>[3x]MHKSAFQALQGDIPTYEVNSSDEQDSDQDEEDVEQPSEPMHRLVSAPAASIHIEESKYISSNFSFDDD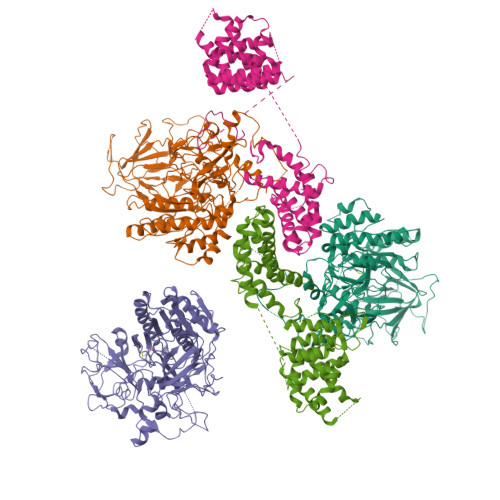NTIYGHDYVIFGLKSNQNLIVKGQFVLEIQRGAIDINGVIYHSGVEPMKFINPSSSSIPLIQATQVLNSSLLENKESQENQHLFTPGYKSVIKLTNLDTHLESIGRVCPLFKNLFWQFDNFFAEDSLRLLDQYELAFSDYTFYPITKPDNTVSVIKHKNWMDVIKSLTELYSNDQSIKVIVIGGKNSGKSTFLRLLVQHMLSPTLQQLPINFMDLDPGQPEYSGTDCISLSKISEVQHGNHLSLTSTDSTQCHYVGFNSPKDQPTRYNLLVEQLVRSYESDGELKHESLLINTPGWIKGYGLELTRTLIERVKPTHVIYLNSGTLGVDIDIPKGTNLIPLQGSFNHSGSRYSSSQLRLLKTMAYFHKIDDFKFDFQPLLFSPPIQVSYGVSTGISALTHLKETGIGMDHLERSIEATIVGIFKVKRDHLEECELFNKGQLPLLPYKEFIKLSTEFFRLALVHSIDQEKKIMNLYIPQFRTLDLTKEAIIMVRGNTDLPIWEIASNEIVKRFKRQLPYITFEKGSSLEKKWKVRKNVQRRGQM;>MNSHPRLTPWKSSDEVVYLKGLFFPADREQISRDELYRQYEEAISLVEMYSSRTRVSHILQSTAHLFSALMMLESFEGGLDDTVRLTASMTIIRFVNGLLDPNQQSQFAIPLHLLAKKIDLPSLFVEFRHSATHDALPSLEMCKTCVDRAIDWVWDHYWDGVLSIVEPQVETDDLEESLIKELKDLFKQYRRIRRQNITKLYKFGDSTPEGKEYWTCIAGIKDHADMANFYNVMIERIVSNKLKWEHLRALFEPMMNHFIHLKGWDFPLGLIDSMLSKNYEYSKFRGIDDTERAYLNDQEFKCAQKWIRWLAIEQIDRYDDVLVSKMIDTLGKTNHELNVELLEKLQSRFSADPVIKDKIQAKLTLIQRLSTDTKTKRMNNLEDIMSDLESLKKRAKVTPTLHIKSFESHPNWTPKPFGVI[3x]>[2x]MGSDKIHHHHHHM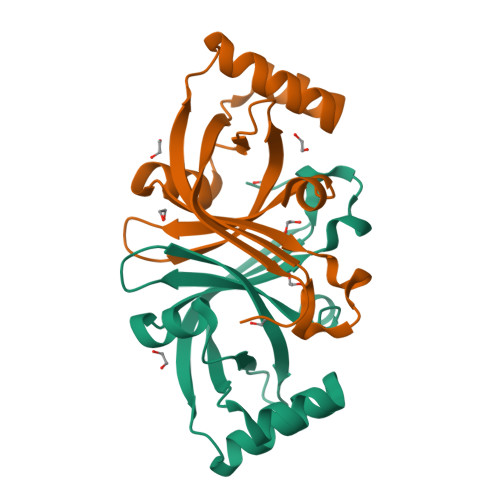SQLEKAQAEYAGFIQEFQSAIISTISEQGIPNGSYAPFVIDDAKNIYIYVSGLAVHTKNIEANPLVNVLFVDDEAKTNQIFARRRLSFDCTATLIERESQKWNQVVDQFQERFGQIIEVLRGLADFRIFQLTPKEGRFVIGFGA>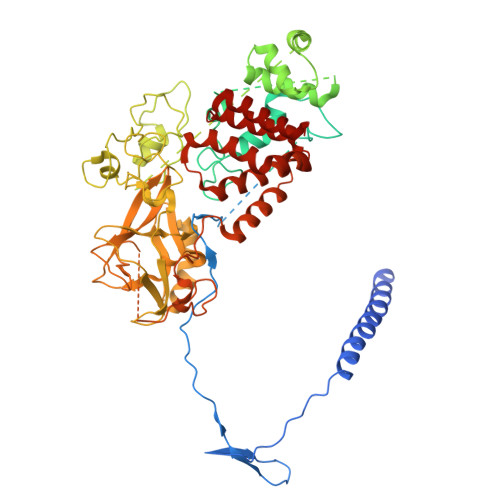 SNAHHHHHHGQTGKKSEKGPVCWRKRVKSEYMRLRQLKRFRRADEVKSMFSSNRQKILERTEILNQEWKQRRIQPVHILTSVSSLRGTRECSVTSDLDFPTQVIPLKTLNAVASVPIMYSWSPLQQNFMVEDETVLHNIPYMGDEVLDQDGTFIEELIKNYDGKVHGDRECGFINDEIFVELVNALGQYNREEKQKDLEDHRDDKESRPPRKFPSDKIFEAISSMFPDKGTAEELKEKYKELTEQQLPGALPPECTPNIDGPNAKSVQREQSLHSFHTLFCRRCFKYDCFLHPFHATPNTYKRKNTETALDNKPCGPQCYQHLEGAKEFAAALTAERIKTPPKRPGGRRRGRLPNNSSRPSTPTINVLESKDTDSDREAGKPNIEPPENVEWSGAEASMFRVLIGTYYDNFCAIARLIGTKTCRQVYEFRVKESSIIAPAPAEDVDTPPRKKKRKHRLWAAHCRKIQLKKDGSSNHVYNYQPCDHPRQPCDSSCPCVIAQNFCEKFCQCSSECQNRFPGCRCKAQCNTKQCPCYLAVRECDPDLCLTCGAADHRDSKNVSCKNCSIQRGSKKHLLLAPSDVAGWGIFIKDPVQKNEFISEYCGEIISQDEADRRGKVYDKYMCSFLFNLNNDFVVDATRKGNKIRFANHSVNPNCYAKVMMVNGDHRIGIFAKRAIQTGEELFFDYRYSQADALKYVGIEREMEIPFLESEDGEVEQQRTYSSGHNRLYFHSDTCLPLRPQEMEVDSEDEKDPEWLREKTITQIEEFSDVNEGEKEVMKLWNLHVMKHGFIADNQMNHACMLFVENYGQKIIKKNLCRNFMLHLVSMHDFNLISIMSIDKAVTKLREMQQKLEKGESAS>[2x]MASMTGGQQMGRGSEFMSSLLVKKLVESATTPMRGSEGAAGYDISSVEDVVVPAMGRIAVSTGISIRVPDGTYGRIAPRSGLAYKYGIDVLAGVIDEDYTGEVKVILYNTTERDYIIKKGDRIAQLILEQIVTPGVAVVLDLSDTARGSGGFGSTGILEHHHHHH

dUTPase (EC 3.6.1.23) is a ubiquitous enzyme that catalyzes the hydrolysis of dUTP to diphosphate and dUMP, the substrate for thymidylate synthetase in dTTP biosynthesis. The 141-amino-acid deoxyuridine triphosphatase (dUTPase) from the algal Chlorella virus IL-3A and its Glu81Ser/Thr84Arg-mutant derivative Mu-22 were crystallized using the hanging-drop vapor-diffusion method at 298 K with polyethylene glycol as the precipitant. We previously generated Mu-22 dUTPase by mutating two IL-3A residues to the corresponding residues from PBCV-1 dUTPase. The presence of these two mutations (Glu81Ser and Thr84Arg), creating the derivative Mu-22 dUTPase, led to an increase in the optimal temperature of the enzyme to 328 K. Here, we conduct structural studies of dUTPases from Chlorella viruses in order to elucidate the molecular mechanisms behind the differences in optimal temperature.

An apo IL-3A dUTPase with an amino-terminal T7 epitope tag and a carboxy-terminal histidine tag yielded cubic P213 crystals with unit-cell parameter a = 106.65 Å.>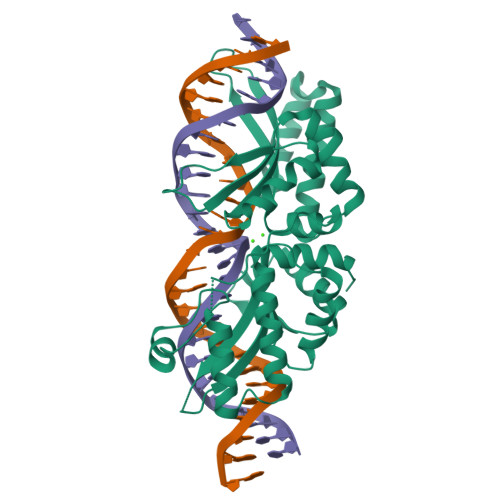 MASSRRESINPWILTGFADAEGSFGLSILNRNRGTARYHTRLSFTIMLHNKDKSILENIQSTWKVGIITNNGDHYVTLRVTRFEDLKVIIDHFEKYPLVTQKLGDYKLFKQAFSVMENKEHLKENGIKELVRIKAKMNWGLNDELKKAFPENISKERPLINKNIPNFKWLAGFTSGDGSFFVRLRKSNVNARVRVQLVFEISQHIRDKNLMNSLITYLGCGHIYEGNKSERSWLQFRVEKFSDINDKIIPVFQENTLIGVKLEDFEDWCKVAKLIEEKKHLTESGLDEIKKIKLNMNKGR> MSRCQNMVD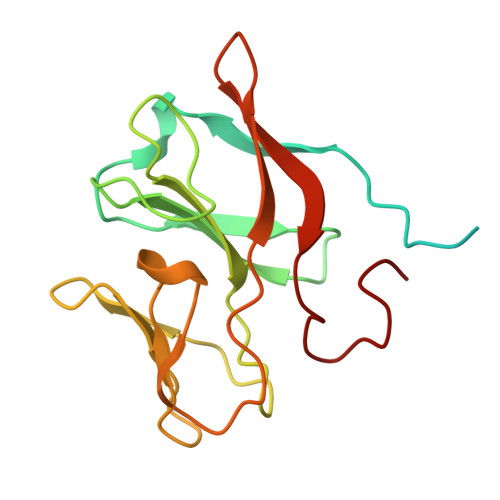IGRRQFLRGGALAAAGATAAVFGVGAPQARAATAAAGVEYPANRLANISELTLNEPLDVAYPDEDAAGVLLKLGTRVEGGVGPDGDIVGFSTICPHKGFPLSYSADNKTFNCPGHFSVFDPEKGGQQVWGQATQNLPQYVLRVADNGDIFAEGVDELIYGRLSNVL> AAEEKTEFDVILKAAGANKVAVIKAVRGATGLGLKEAKDLVESAPAALKEGVSKDD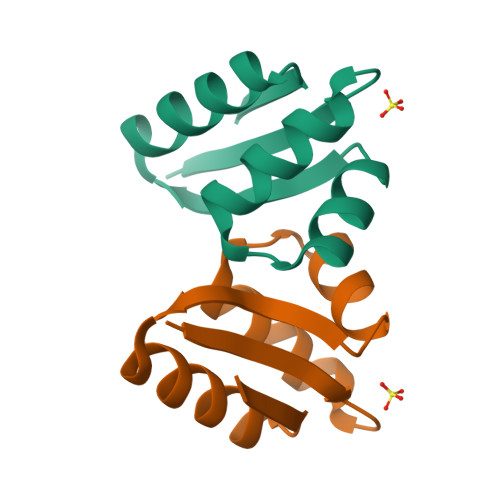AEALKKALEEAGAEVEVK>[4x]XXXXXXXKLANVVILATGGTIAGAGASAANSATYQAAKVGVDKLIAGVPELADLANVRGEQVMQIASESITNDDLLKLGKRVAELADSNDVDGIVITHGTDTLEETAYFLDLTLNTDKPIVVVGSMRPGTAMSADGMLNLYNAVAVASNKDS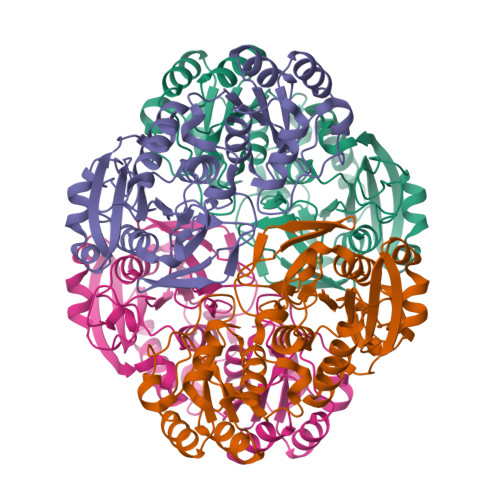RGKGVLVTMNDEIQSGRDVSKSINIKTEAFKSAWGPLGMVVEGKSYWFRLPAKRHTVNSEFDIKQISSLPQVDIAYSYGNVTDTAYKALAQNGAKALIHAGTGNGSVSSRLTPALQTLRKTGTQIIRSSHVNQGGFVLRNAEQPDDKNDWVVAHDLNPEKARILVELAMVKTQDSKELQRIFWEY>MYGKLNKLVEHIKELLQQLNKNWHRLQSNLHDMLQQMEQLFQEFQHFMQGNQDDGKLQNMIHEMQQFMNQLDNHLQSLSDTVHHFHNKLQELMNNFH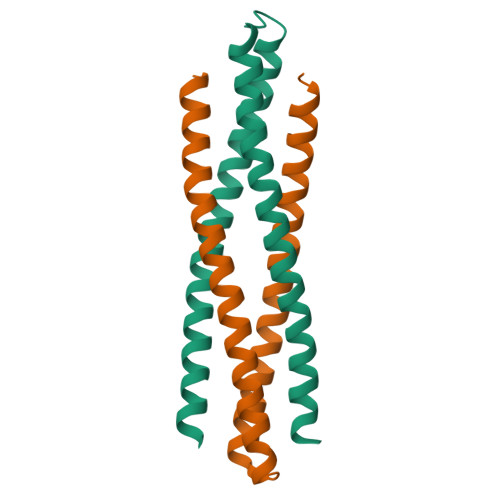HLVHK[4x]> GLTSCEIDNYEGPDASIHGSILDEQTGELVGSDMENGNAIKVREHGFTNATDQTWYITNTGEYRNNMVFAATYDVRFENGNFYPFEVKDF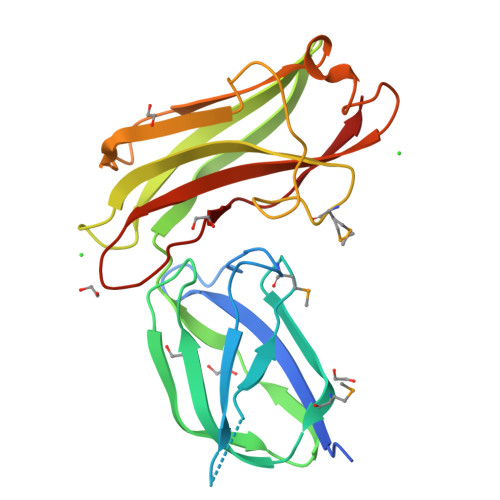VVKSGDNVYDFKVIPYIRVKSPKVEKNGNVITATFSLEAGKQEVKLKEIQLFAFSDMWVGNNVKLTLNGGTDKQVFSPSTAINSADIYTLSIDLGQNADVLKYSKNYYFRIGALADVSGVGTVRHNYAPVVVIKL methyl (2R,7S)-7-({(2E)-3-[5-chloro-2-(1H-tetrazol-1-yl)phenyl]prop-2-enoyl}amino)-14-[(methoxycarbonyl)amino]-2,3,4,5,6,7-hexahydro-1H-8,11-epimino-1,9-benzodiazacyclotridecine-2-carboxylate | C29 H30 Cl N9 O5 | 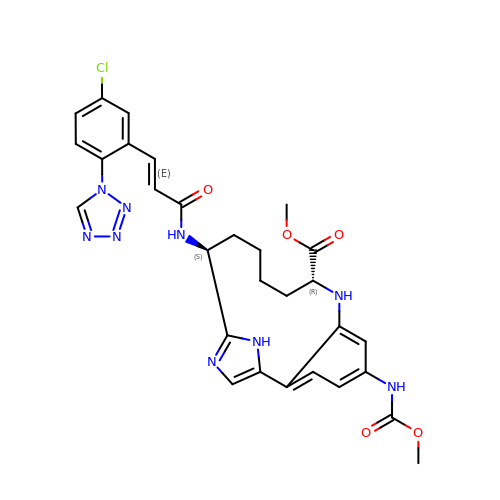IMAMZDHZESKXTJ-VFPWRSFOSA-N>TNQCTVRYNVADCSHLKLTHIPDDLPSNITVLNLTHNQLRRLPPTNFTRYSQLAILDAGFNSISKLEPELCQILPLLKVLNLQHNELSQISDQTFVFCTNLTELDLMSNSIHKIKSNPFKNQKNLIKLDLSHNGLSSTKLGTGVQLENLQELLLAKNKILALRSEELEFLGNSSLRKLDLSSNPLKEFSPGCFQTIGKLFALLLNNAQLNPHLTEKLCWELSNTSIQNLSLANNQLLATSESTFSGLKWTNLTQLDLSYNNLHDVGNGSFSYLPSLRYLSLEYNNIQRLSPRSFYGLSNLRYLSLKRAFTKQSVSLASHPNIDDFSFQWLKYLEYLNMDDNNIPSTKSNTFTGLVSLKYLSLSKTFTSLQTLTNETFVSLAHSPLLTLNLTKNHISKIANGTFSWLGQLRILDLGLNEIEQKLSGQEWRGLRNIFEIYLSYNKYLQLSTSSFALVPSLQRLMLRRVALKNVDISPSPFRPLRNLTILDLSNNNIANINEDLLEGLENLEILDFQHNNLARLWKRANPGGPVNFLKGLSHLHILNLESNGLDEIPVGVFKNLFELKSINLGLNNLNKLEPFIFDDQTSLRSLNLQKNLITSVEKDVFGPPFQNLNSLDMRFNPFDCTCESISWFVNWINQTHTNISELSTHYLCNTPHHYYGFPLKLFDTSSCKDSAPFEL[4x]

Toll-like receptor 3 (TLR3) is a member of the TLR family, which plays an important role in the innate immune system and is responsible for recognizing viral double-stranded RNA (dsRNA). TLR3 primarily localizes to endolysosome and is activated by double-stranded RNAs (dsRNAs) released from viruses or necrotic cells during viral infection or inflammation. The structure of TLR3 complexed with dsRNA reveals that the two protomers of TLR3 sandwich the dsRNA, interacting with the ribose phosphate backbone of dsRNA with no apparent sequence specificity. TLR3 dimers laterally form a higher multimeric complex along dsRNA, providing the basis for cooperative binding and efficient signal transduction.

Therefore, we performed cryo-EM analysis of TLR3 complexed with 90 bp dsRNA, which was designed to accommodate two dimer units of TLR3. Subsequently, we collected cryo-EM images using stage tilts (0°, 30°, and 40°) and reconstructed a cryo-EM map of TLR3 complexed with 90 bp dsRNA at a resolution of 3.2 Å. Although the stage tilts partially improved the particle orientations, the map was not of high quality due to the lack of information from missing directions; however, it was sufficient for locating the four TLR3 molecules and most regions of the 90 bp dsRNA (81 bp). The cryo-EM structure showed that the dimeric TLR3 units were aligned laterally to dsRNA (dimers A and B). The two dimers were related by a translational shift of approximately 90 Å, corresponding to three turns of the dsRNA without any rotation around it. In total, the width of the tetramer was approximately 240 Å, covering approximately 80 bp of the dsRNA. The protomers from the dimeric unit on the same side of dsRNA are proximal to each other in a head-to-tail arrangement (TLR3A and TLR3B, and TLR3A* and TLR3B*, wherein the partner TLR3 is denoted with asterisks). The residues in C-terminal region are negatively charged (E524, D525, and E528 [LRR19]), and those in the N-terminal region are positively charged (K138, K140, K145, and K148 [LRR4], and K164 [LRR5]). Since electrostatic forces reach far in distance, we hypothesized that the electrostatic interactions between two TLR3 dimeric units facilitate higher-order oligomer formation of TLR3 along dsRNA laterally, possibly resulting in efficient signal transduction. Thus, its tetramer structure along 90 bp dsRNA is a representative model for the lateral multimerization of TLR3 along longer dsRNAs.> MKTLVHVASVEKGRSYEDFQKVYNAIALKLREDDEYDNYIGYGPVLVRLAWHISGTWDKHDNTGGSYGGTYRFKKEFNDPSNAGLQNGFKFLEPIHKEFPWISSGDLFSLGGVTAVQEMQGPKIPWRCGRVDTPEDTTPDNGRLPDYDKDAGYVRTFFQRLNMNDREVVALMGAHALGKTHLKNSGYEGPWGAANNVFTNEFYLNLLNEDWKLEKNDANNEQWDSKSGYM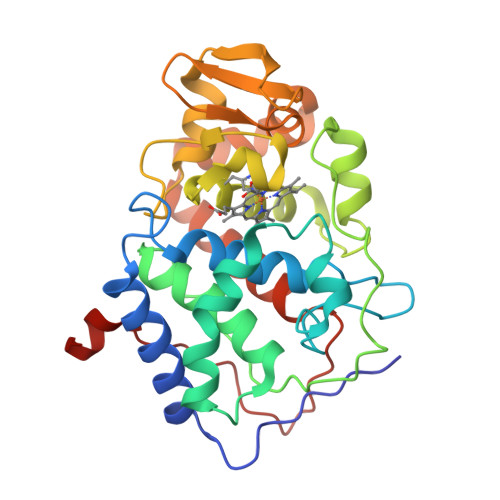MLPTDYSLIQDPKYLSIVKEYANDQDKFFKDFSKAFEKLLENGITFPKDAPSPFIFKTLEEQGL> MIRGSSALKSLTSRRLYSTGVKYTTLSNGVTVATETNPAAKTSSVGLFFGAGSRSEHSHSNGISALTTNVLASQSAKGSLLTAKNDREFNGIIAQTTNDNITEAGKLIASIASNAVDIVEKTDLTKHKQYLSAQASAVEADPKSKVLSHLYSSAFQGYSLALPTLGTTESVENLENQDSLRHLAKHLVNNNTVIAASGNFDHDKLADAIEANLKIAEGVKPEIKPASFLGSEVRMRDDTLPKAYISIAVHGEGLNSPNYYLAKVAAA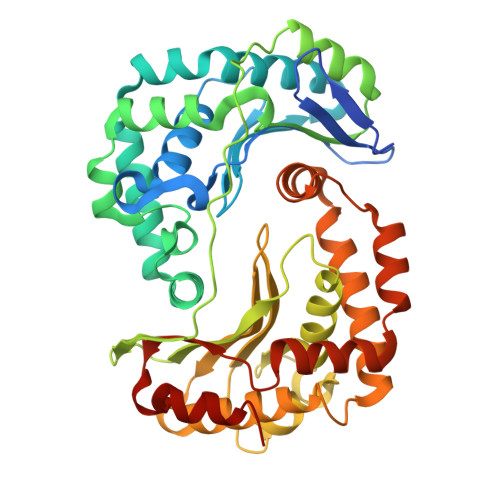IYGDFYLHSTIAKFTSPKLASIVQEYNIVESYNHYSKSFSDTGIWGYYAEIADKFTVDDFTHFSLKEWNRLSISISEAEVARAKAQVKTALAKELANSFAVTSDIAEKVLLVGHRQSLREAFEKIDAIKVNDVKEWGKSKVWDRDIVISGTGLIEDLLDYNRNRNEMAMMRW>[2x]MSARMDNDTAALLERIRSDWARLNHGQGPDSDGLTPSAGPMLTLLLLQRLHAALGREIERTYAASGLNAAGWDLLLTLYRSAPPEGLRPTELSALAAIS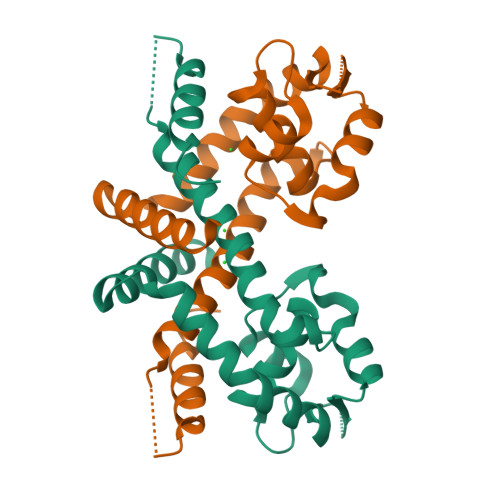GPSTSNRIVRLLEKGLIERREDERDRRSASIRLTPQGRALVTHLLPAHLATTQRVLAPLSAQEQRTLEELAGRMLAGLEQGV> MKTITLYLDPASLPALNQLMDFTQNNEDKTHPRIFGLSRFKIPDNIITQYQNIHFVELKDNRPTEALFTILDQYPGNIELNIHLNIAHSVQLIRPILAYRFKHLDRVSIQQLNLYDDGSDEYVDLEKEENKDISAEIKQAEKQLSHYLLTGKIKFDNPTIARYVWQSAFPVKYHFLSTDYFEKAEFLQPLKEYLAENYQKMDWTAYQQLTPEQQAFYLTLVGFNDEVKQSLEVQQAKFIFTGTTTWEGNTDVREYYAQQQLNLLNHFTQAEGDLFIGDHYKIYFKGHPRGGEINDYILNNAKNITNIPANISFEVLMMTGLLPDKVGGVASSLYFSLPKEKISHIIFTSNKQVKSKEDALNNPYVKVMR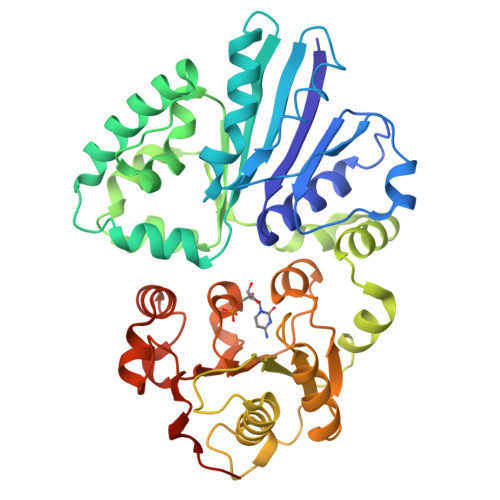RLGIIDESQVIFWDSLKQLGGGLEHHHHHH>PPGPPGPPGPRXPPGPPGPPGPP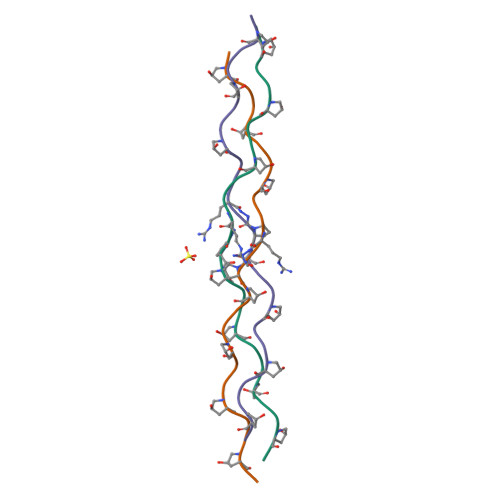GX[3x]> TWGVSSPKNVQGLSGSCLLIPCIFSYPADVPVSNGITAIWYYDYSGKRQVVIHSGDPKLVDKRFRGRAELMGNMDHK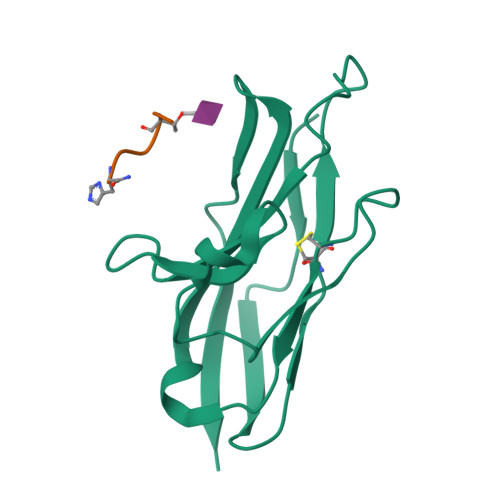VCNLLLKDLKPEDSGTYNFRFEISDSNRWLDVKGTTVTVTT;> AGHTWGH Rebamipide | 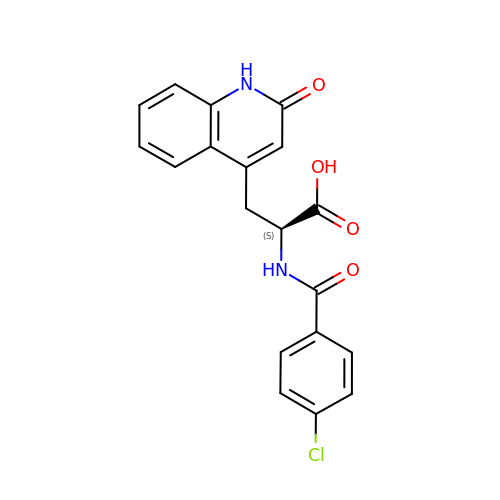C19 H15 Cl N2 O4 | ALLWOAVDORUJLA-INIZCTEOSA-N1,3-benzoxazine-2,4-dione 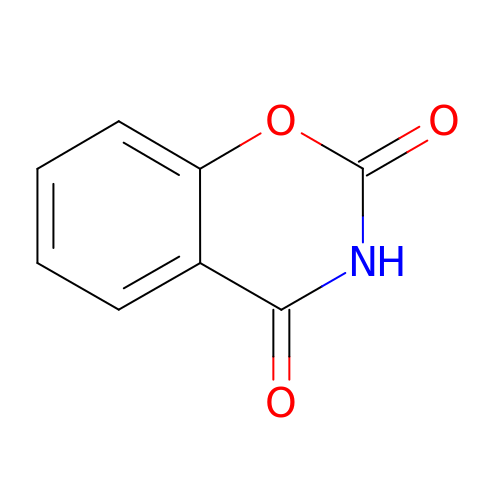| C8 H5 N O3 | OAYRYNVEFFWSHK-UHFFFAOYSA-N>FVVSEAQFDQMFPSRNSFYTYSGL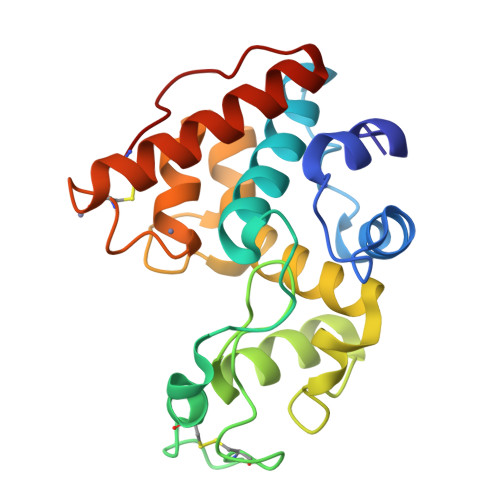TAALSAYPGFSNTGSDTVKKQEAAAFLANVGHETGGLVYVVEQNTANYPHYCDASQPYGCPAGNDKYYGRGPVQLSWNFNYKAAGDALGIDLLNNPDLVQNDSAVAWKTGLWYWNTQTGPGTMTPHDAMVNGAGFGETIRSINGSLECDGGNPGQVQSRIDNYERFTQLLGVEPGGNLSC[2x]>REKFFGDQVLRINVRNGDEISKLSQLVNSNNLKLNFWKSPSSFNRPVDVLVPSVSLQAFKSFLRSQGLEYAVTIEDLQALLDNEDDEMQHNEGQERSSNNFNYGAYHSLEAIYHEMDNIAADFPDLARRVKIGHSFENRPMYVLKFSTGKGVRRPAVWLNAGIHSREWISQATAIWT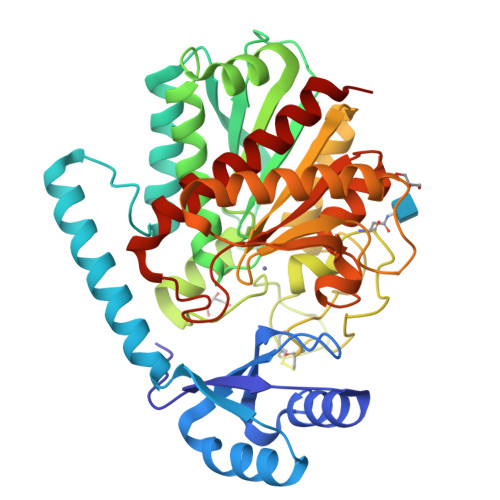ARKIVSDYQRDPAITSILEKMDIFLLPVANPDGYVYTQTQNRLWRKTRSRNPGSSCIGADPNRNWNASFAGKGASDNPCSEVYHGPHANSEVEVKSVVDFIQKHGNFKGFIDLHSYSQLLMYPYGYSVKKAPDAEELDKVARLAAKALASVSGTEYQVGPTCTTVYPASGSSIDWAYDNGIKFAFTFELRDTGTYGFLLPANQIIPTAEETWLGLKTIMEHVRDNLY[2x]>MHHHHHHDPPCEELEIVWKNIKAEARALADCEPMLASFYHATLLKHENLGSALSYMLANKLASPIMPAIAIREVVEEAYAADPEMIASAACDIQAVRTRDPAVDKYSTPLLYLKGFHALQAYRIGHWLWNKGRRALAIFLQNQVSVSFQVDIHPAAKIGRGIMLDHATGIVVGETAVIEDDVSILQSVTLGGTGKTSGDRHPKIRE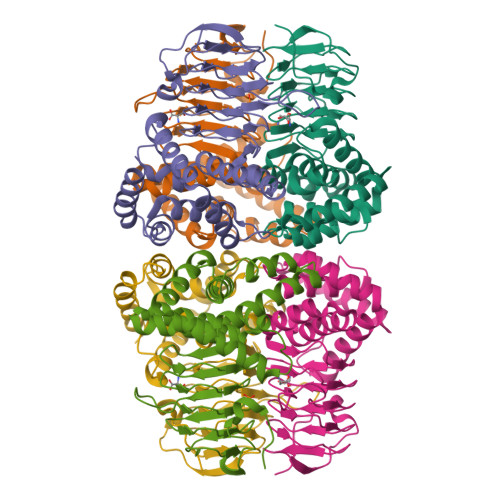GVMIGAGAKILGNIEVGRGAKIGAGSVVLQPVPPHTTAAGVPARIVGKPGSDKPSMDMDQHFNGIHHTFEYGDG[3x]N-glycolyl-beta-neuraminic acid | C11 H19 N O10 | 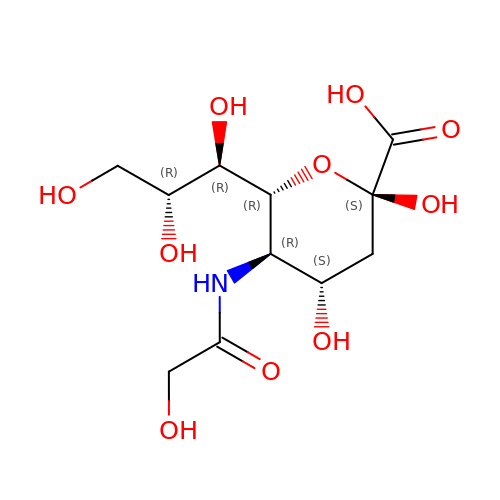FDJKUWYYUZCUJX-AJKRCSPLSA-N> KDDKVASATDVQFETPLKIVEYPDPILRAKNKRIDIFDENLKNLVDAMFDVMYKTDGIGLSAPQVGLNVQLMVFNPAGEPGEGKEIVLVNPKIKKYSDKLVPFDEGCLSFPGIYAEVVRPQSVKIDARD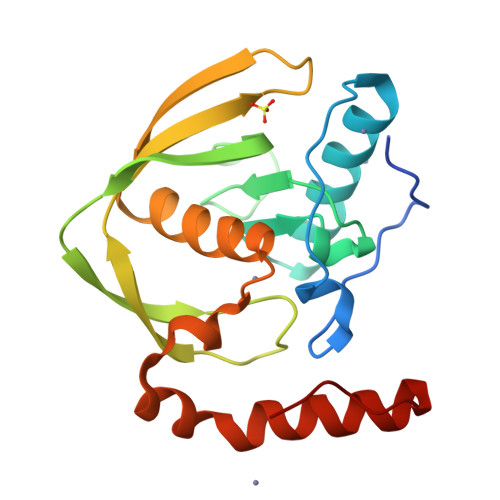ITGERFSISLSRLPARIFQHEYDHLEGVLFFDRMTDQVLDSIREELEALEKKYEEKTGLPSPER>MSSIKVECVLRENYRCGESPVWEEASQSLLFVDIPSKIICRWDTVSNQVQRVAVDAPVSSVALRQLGGYVATIGTKFCALNWENQSVFVLAMVDEDKKNNRFNDGKVDPAGRYFAGTMAEETAPAVLERHQGSLYSLFPDHSVKKYFDQVDISNGLDWSLDHKIFYYIDSLSYTVDAFDYDLQTGQISNRRIVYKMEKDEQIPDGMCIDAEGKLWVACYNGGRVIRLDPETGKRLQTVKLPVDKTTSCCFGGKDY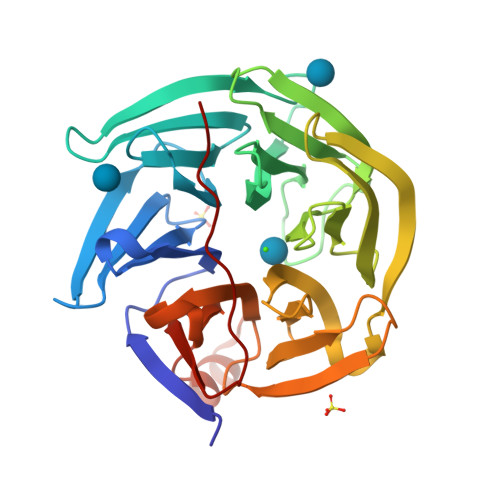SEMYVTCARDGLNAEGLLRQPDAGNIFKITGLGVKGIAPYSYAG[2x]N-methylpyrimidine-2-carboximidamide | C6 H8 N4 | 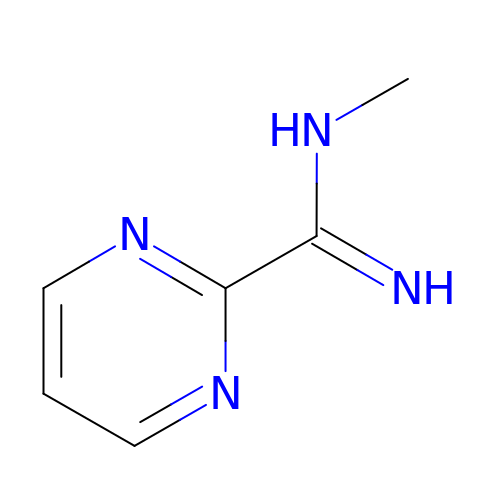GXUPAQKJNPTPOU-UHFFFAOYSA-N> SHVPYKVVRTPSGNLPVYSRVRKHGTEVTTIVRHAFGDITAMK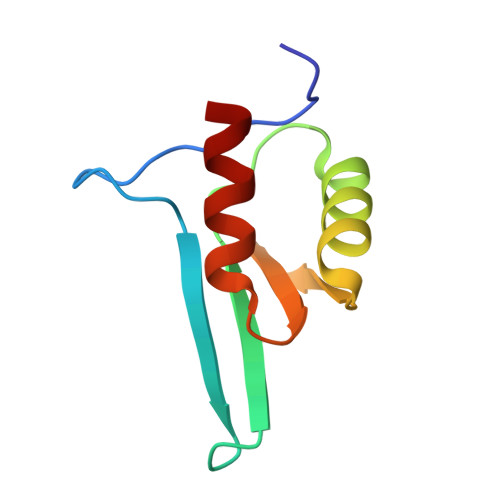KDLVAICEAPVRERLGTLEVKGLHVLKIKQWLRSLG> AYTTFSQTKNDQLKEPMFFGQPVNVARYDQQKYDIFEKLIEKQLSFFWRPEEVDVSRDRIDYQALPEHEKHIFISNLKYQTLLDSIQGRSPNVALLPL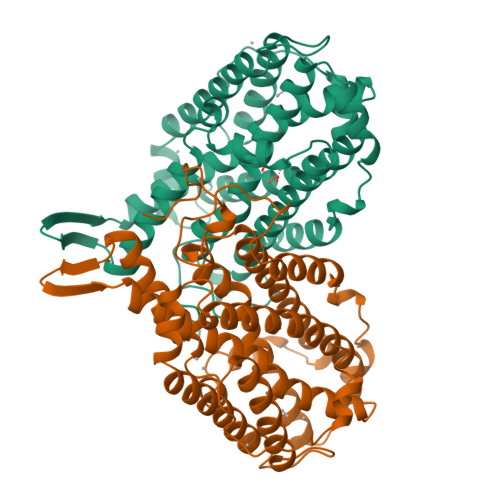ISIPELETWVETWAFSETIHSRSFTHIIRNIVNDPSVVFDDIVTNEQIQKRAEGISSYYDELIEMTSYWHLLGEGTHTVNGKTVTVSLRELKKKLYLCLMSVNALEAIRYYVSFACSFAFAERELMEGNAKIIRLIARDAALHLTGTQHMLNLLRSGADDPEMAEIAEECKQECYDLFVQAAQQEKDWADYLFRDGSMIGLNKDILCQYVEYITNIRMQAVGLDLPFQTRSNPIPWINTWLVSDNVQVAPQEVEVSSYLVGQIDSEVDTDDLSNFQL;> AYTTFSQTKNDQLKEPMFFGQPVNVARYDQQKYDIFEKLIEKQLSFFWRPEEVDVSRDRIDYQALPEHEKHIFISNLKYQTLLDSIQGRSPNVALLPLISIPELETWVETWAFSETIHSRSFTHIIRNIVNDPSVVFDDIVTNEQIQKRAEGISSYYDELIEMTSYWHLLGEGTHTVNGKTVTVSLRELKKKLYLCLMSVNALEAIRFYVSFACSFAFAERELMEGNAKIIRLIARDAALHLTGTQHMLNLLRSGADDPEMAEIAEECKQECYDLFVQAAQQEKDWADYLFRDGSMIGLNKDILCQYVEYITNIRMQAVGLDLPFQTRSNPIPWINTWLVSDNVQVAPQEVEVSSYLVGQIDSEVDTDDLSNFQL>MEHKRGHVLAVPYPTQGHITPFRQFCKRLHFKGLKTTLALTTFVFNSINPDLSGPISIATISDGYDHGGFETADSIDDYLKDFKTSGSKTIADIIQKHQTSDNPITCIVYDAFLPWALDVAREFGLVATPFFTQPCAVNYVYYLSYINNGSLQLPIEELPFLELQDLPSFFSVSGSYPAYFEMVLQQFINFEKADFVLVNSFQELELHENELWSKACPVLTIGPTIPSIYLDQRIKSDTGYDLNLFESKDDSFCINWLDTRPQGSVVYVAFGSMAQLTNVQMEELASAVSNFSFLWVVRSSEEEKLPSGFLETVNKEKSLVLKWSPQLQVLSNKAIGCFLTHCGWNSTMEALTFGVPMVAMPQWTDQPMNAKYIQDVWKAGVRVKTEKESGIAKREEIEFSIKEVMEGERSKEMKKNVKKWRDLAVKSL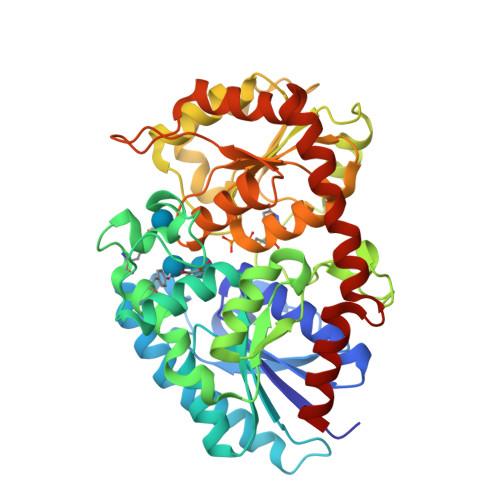NEGGSTDTNIDTFVSRVQSK[2x]>MAQLTQMTNEQLRE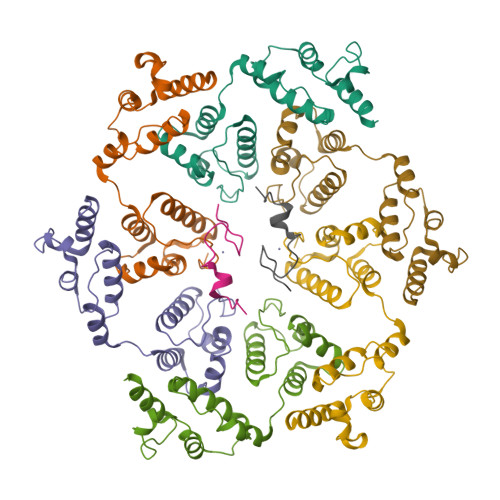LIEAVRAAAVGAAGSAAAAGGADASRGKGNFSACTHSFGGTRDHDVVEEFIGNIETYKDVEGISDENALKGISLLFYGMASTWWQGVRKEATTWKEAIALIREHFSPTKPAYQIYMEFFQNKQDDHDPIDTFVIQKRALLAQLPSGRHDEETELDLLFGLLNIKYRKHISRHSVHTFKDLLEQGRIIEHNNQEDEEQLATAKNTRGSKRTTRCTYCSFRGHTFDNCRKRQKDRQEEQHEE[8x]> MESQDIDYLKFNDFKSDIEDFEIGQDISGYDNSKIDFDSNVITISNEYGILLIVSPELNDLLVTPIEGLLNYIQSNDQDTNDQTTILSCPTIIKVGKVFEIPSSTKTSFKINLLFSPNGDYFSISYHKTLKVYSTKDSISKKWVNIKPIVEINGKFDSNIASTKWNHSNDTIAVVTANSSLFFVSIGNGSLNKIEEPAVDVCWDVKKSKQIYVALEDSSIILIDSSKPGHEIFRIENPITNYEDEDEEEEELNYYVSSINLVADEFLLVQYYIVRMDEYEDSPAFLFDLKDDESKSQEFQLSIMPEGNFQSAIHLASSFIKDWNLLIVCSNKGMGPDLLQLDTKTREWKTLKLEDEFGITLPNPVVLGMQLITCYPTQPKNLNGIQKYTTNGTFPPVPILLIVDDSAHFKFSNLFNINSKNLSIIQSPKSIQQQQQQQQQEQQQQQQTPSLFQSQTPSLFQQQKPQQPSSSLFQTTQTPAPSLFQQPQQTPTTSIFQQPKAPTTSIFQQQQQAPTTSIFQQQQQSPTTSILQQQQAPTTSIFQQQQQQQQSTQQQQKPKTIPTISPIKSMSTTFTNSVSTAPSQKQQQPSQQPSQQQQSQQQPFKRQNSAPTPISTPISTPIKNELSGNSNVYPNSTLKKYMQKIENTSNVYNGQSPISQQIRKNLKSIENYYQAIRRNSIEGNKIHQTIKNGFLANHQNTKTEIEEFQQSINSLTTEFKKNDKQSSLLKSQVLKNLSLSLDLESHTQQYSSTNYKQILANRNLDPSTLEQKDKLLSNYRNLSLDIQNFEQTHFKFLENNQNNQNNQNNIEKVHINSMSLIYQSLSNISQTETNLRCEIEKIEKKLNKLKLNKDKMDRLKDSIDINQYTELQLSRLSLENNVNILNDNGSGKDIKSTTKPTIENYRHEVNVSKSNGYKNLISVLKRKSSQVIKPQYPDFTSFFKSEQIDDPQFDDDIINNEYNNNNNNNSEIIEPPPALRGISLSKDNAFANSSYKFTSNITPIKTSGTISSPSSTTSSFTPTSHISFASTAQNFINNNQSYDDYQDGNEEYDEDDDDDDEQYDEDDEEYIEEPINPIPSLNKQQPQQQ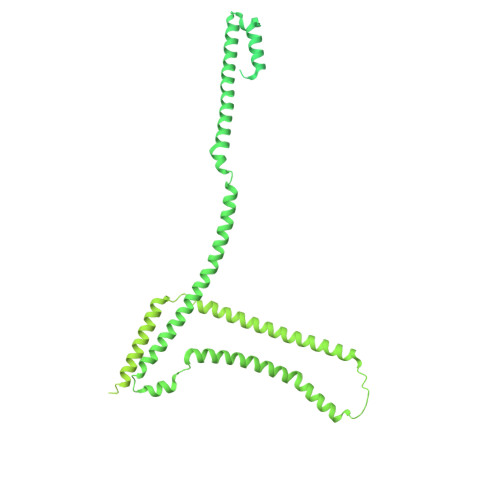QQFGNNNNFGNLFNSQQPTNSNSLFTKNLDLEKEAKERQEKIERETRELQDKLEREEREAKEKQARELKDKLEREAKEKQARELKEKQEREAKEKAEKEANEKQEREAKEKAEKEAREKIEKEAKEKLEREAKEKLEREAKEKAEKEAKEKLEKEAKEKLEKEAKEKAEKDSANANNALGALNFGGNTTSTASGSSPFGSGGLFGTTTTPTTTAATPTPPSVFGGNSASTTTGGGSIFSQASTNSPPSPFGGSVFGAKPAPQTSSVFGSAPSTASAFGGSTTTSSFGATTATPTPFGGGGSVFGAKPAPQTSSVFGSTSSPSTTTSAFGSTSTTPSVFGNTSAFGGGGSTTTPTTSAFGSSSTTPAFGGTPAFGSAPTTSAFGSAPTTTTSAFGSSSTPAFGGTSAFGSAPTTSAFGSTPATGAFGSAPTTSAFGSTPATSAFGSTPTTGAFGSTPTTGAFGSTPTTSAFGSTPTTGAFGSTPTTSAFGSTSAFGSTPTTSAFGGAPTTNAFGSSSTPAFGSTPTTSAFGSSSTPAFGGTSAFGGAPTTSAFGSSSTPAFGGTSAFGSTPTTSAFGGGSVFGSTSSQPTSSVFGSQFGSNSAPSFASLGGGSFGK>[2x]MEHHHHHHNKDLKGLYAALLVPFDENGQVNEQGLKQIAQNAIETEELDGLYVNGSSGENFLLNTEQKKQVFKVAKEAVGDKVKLIAQVGSLDLNEAIELGKYATELGYDALSAVTPFYYPFTFEEIRDYYFDIIEATQNNMIIYAIPDLTGVNISIEQFSELFNHEKIVGVKYTAPNFFLLERIRKAFPDKLILSGFDEMLVQATISGVDGAIGSTYNVNGRRARKIFDLARQGQIQEAYQLQHDSNDIIETVLSMGIYPTLKEILRHRGIDAGLPKRPFKPFNEAHRQTLDQLIAKYDL

N-Acetyl neuraminic acid lyase (NAL) is a Class I aldolase that catalyses the reversible aldol reaction between pyruvate and N-acetyl mannosamine (ManNAc) to give N-acetyl neuraminic acid (Neu5Ac). The catalysis of reactions involving fluoropyruvate as donor by N-acetyl neuraminic acid lyase (NAL) variants was investigated. Despite a report that it is not a substrate, fluoropyruvate is a viable donor. A combination of mutagenesis, structural biology and computational chemistry has revealed insights into its catalytic mechanism.

The crystal structure of S. aureus NAL in complex with fluoropyruvate was determined, assisting rationalisation of the stereochemical outcome of C–C bond formation. The crystal structure of S. aureus NAL in complex with fluoropyruvate reveals the presence of a (Z)-configured enamine. The formation of a Z-configured enamine was observed, which presents only one face to aldehyde substrates. Reaction of this face of the (Z)-enamine intermediate would necessarily lead to the formation of 3R-configured products. The (3R)-selectivity of NAL catalysed reactions may be rationalised in terms of selective reaction of this (Z)-configured enamine via the face that is presented to aldehyde substrates. Previous studies have shown that an analogue of DHOB – (2R,3S)-2,3-trihydroxy-4-oxo-N,N-dipropyl butanamide – can bind to the E192N variant of E. coli NAL in two distinct conformations.15 Aldehyde substrates may react via conformations that allow protonation by the general acid Y137.10 The facial selectivity of the reaction of the aldehyde determines the configuration of the product – (3R,4R) or (3R,4S) – obtained. Wild-type NAL catalysed the reaction between fluoropyruvate and ManNAc, albeit much less efficiently than with pyruvate as donor. Under kinetic control, the wild-type enzyme catalysed the reaction between fluoropyruvate and N-acetyl mannosamine to give a 90 : 10 ratio of the (3R,4R)- and (3S,4R)-configured products; after extended reaction times, equilibration occurred to give a 30 : 70 mixture of these products.> GLPVLNTPGSNQFMTSDDFQSPSAMPQFDVTPHMDIPGEVHNLMEIAEVDSVVPVNNIKANLQSMDAYHIEVNTGNYQGEKIFAFQMQPGLESVFKRTLMGEILNYYAHWSGSIKLTFTFCGSAMATGKLLLAYSPPGADVPATRKQAMLGTHMIWDIGLQSSCVLCIPWISQTHYRLVQQDE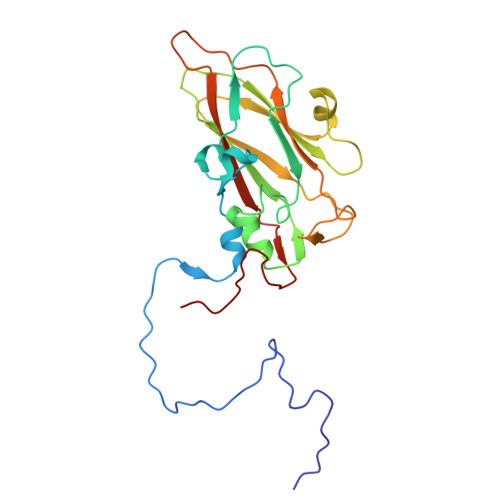YTSAGNVTCWYQTGIVVPPGTPNKCVVLCFASACNDFSVRMLRDTPFIGQTALLQ> GSDNESDEEVAGKKSFSAQEREYIRQGKEATAVVDQILAQEENWKFEKNNEYGDTVYTIEVPFHGKTFILKTFL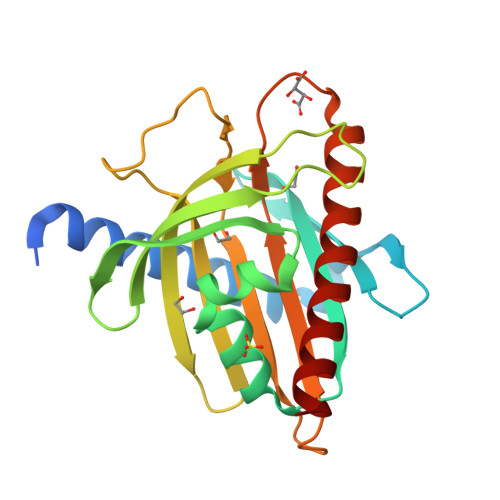PCPAELVYQEVILQPERMVLWNKTVTACQILQRVEDNTLISYDVSAGAAGGVVSPRDFVNVRRIERRRDRYLSSGIATSHSAKPPTHKYVRGENGPGGFIVLKSASNPRVCTFVWILNTDLKGRLPRYLIHQSLAATMFEFAFHLRQRISELGAR> MSRKQLALFEPTLVVQALKEAVKKLNPQAQWRNPVMFIVWIGSLLTTCISIAMASGAMPGNALFSAAISGWLWITVLFANFAE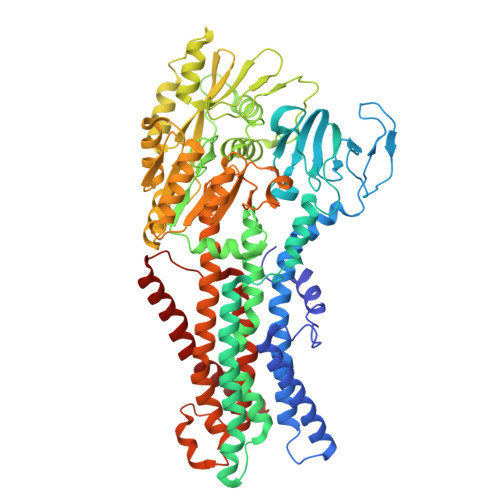ALAEGRSKAQANSLKGVKKTAFARKLREPKYGAAADKVPADQLRKGDIVLVEAGDIIPCDGEVIEGGASVDESAITGESAPVIRESGGDFASVTGGTRILSDWLVIECSVNPGETFLDRMIAMVEGAQRRKTPNEIALTILLIALTIVFLLATATLWPFSAWGGNAVSVTVLVALLVCLIPTTIGGLLSAIGVAGMSRMLGANVIATSGRAVEAAGDVDVLLLDKTGTITLGNRQASEFIPAQGVDEKTLADAAQLASLADETPEGRSIVILAKQRFNLRERDVQSLHATFVPFTAQSRMSGINIDNRMIRKGSVDAIRRHVEANGGHFPTDVDQKVDQVARQGATPLVVVEGSRVLGVIALKDIVKGGIKERFAQLRKMGIKTVMITGDNRLTAAAIAAEAGVDDFLAEATPEAKLALIRQYQAEGRLVAMTGDGTNDAPALAQADVAVAMNSGTQAAKEAGNMVDLDSNPTKLIEVVHIGKQMLMTRGSLTTFSIANDVAKYFAIIPAAFAATYPQLNALNIMCLHSPDSAILSAVIFNALIIVFLIPLALKGVSYKPLTASAMLRRNLWIYGLGGLLVPFIGIKVIDLLLTVCGLV ETHYL (4R)-4-[(TERT-BUTOXYCARBONYL)AMINO]-5-[(3S)-2-OXOPYRROLIDIN-3-YL]PENTANOATE | C16 H28 N2 O5 | 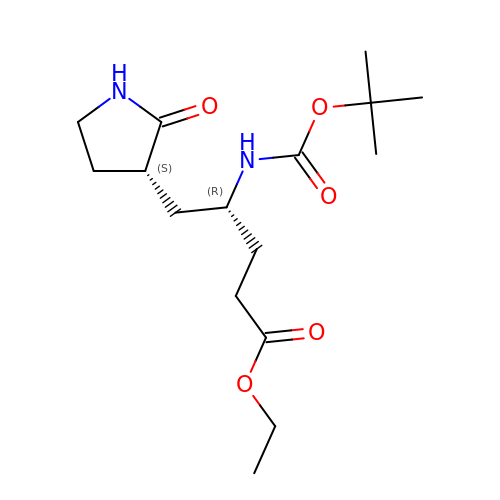VOUMGEIBLJTQJX-NWDGAFQWSA-N> KVFERCELARTLKRLGMDGYRGVSLANWMCLAKWESGYNTRATNYNAGDRSTDYGIFQINSRYWCNDGKTP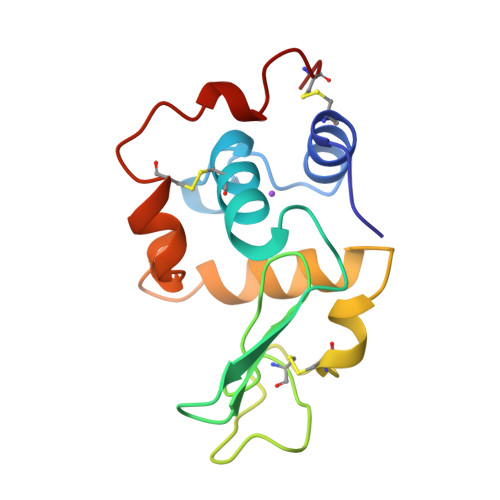GAVNAAHLSCSALLQDNIADAVAAAKRVVRDPQGIRAWVAWRNRCQNRDVRQYVQGCGV> MRGSHHHHHHGSLVPRGSPFVNKQFNYKDPVNGVDIAYIKIPNAGQMQPVKAFKIHNKIWVIPERDTFTNPEEGDLNPPPEAKQVPVSYYDSTYLSTDNEKDNYLKGVTKLFERIYSTDLGRMLLTSIVRGIPFWGGSTIDTELKVIDTNCINVIQPDGSYRSEELNLVIIGPSADIIQFECKSFGHEVLNLTRNGYGSTQYIRFSPDFTFGFEESLEVDTNPLLGAGKFATDPAVTLAHQLIHAGHRLYGIAINPNRVFKVNTNAYYEMSGLEVSFEELRTFGGHDAKFIDSLQENEFRLYYYNKFKDIASTLNKAKSIVGTTASLQYMKNVFKEKYLLSEDTSGKFSVDKLKFDKLYKMLTEIYTEDNFVKFFKVLNAKTFLNFDKAVFKINIVPKVNYTIYDGFNLRNTNLAANFNGQNTEINNMNFTKLKNFTGLFEFYKLLCVRGIITSKTKSLDKGYNKALNDLCIKVNNWDLFFSPSEDNFTNDLNKGEEITSDTNIEAAEENISLDLIQQYYLTFNFDNEPENISIENLSSDIIGQLELMPNIERFPNGKKYELDKYTMFHYLRAQEFEHGKSRIALTNSVNEALLNPSRVYTFFSSDYVKKVNKATEAAMFLGWVEQLVYDFTDETSEVSTTDKIADITIIIPYIGPALNIGNMLYKDDFVGALIFSGAVILLEFIPEIAIPVLGTFALVSYIANKVLTVQTIDNALSKRNEKWDEVYKYIVTNWLAKVNTQIDLIRKKMKEALENQAEATKAIINYQYNQYTEEEKNNINFNIDDLSSKLNESINKAMININKFLNQCSVSYLMNSMIPYGVKRLEDFDASLKDALLKYIYDNRGTLIGQVDRLKDKVNNTLSTDIPFQLSKYVDNQRLLSTFTEYIKNIINTSILNLRYESNHLIDLSRYASKINIGSKVNFDPIDKNQIQLFNLESSKIEVILKNAIVYNSMYENFSTSFWIRIPKYFNSISLNNEYTIINCMENNSGWKVSLNYGEIIWTLQDTQEIKQRVVFKYSQMINISDYINRWIFVTITNNRLNNSKIYINGRLIDQKPISNLGNIHASNNIMFKLDGCRDTHRYIWIKYFNLFDKELNEKEIKDLYDNQSNSGILKDFWGDYLQYDKPYYMLNLYDPNKYVDVNNVGIRGYMYLKGPRGSVMTTNIYLNSSLYRGAKFIIKKYASGNKDNIVRNNDRVYINVVVKNKEYRLATNASQAGVEKILSALEIPDVGNLSQVVVMKS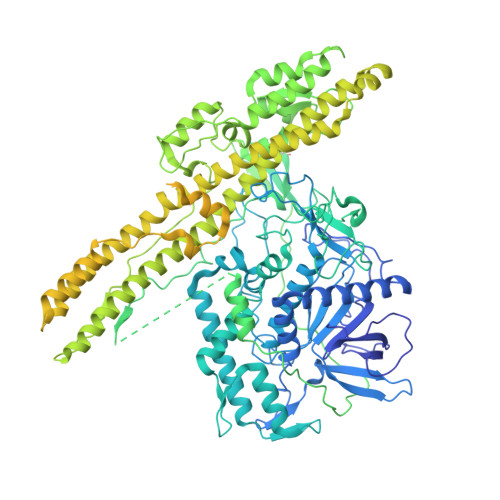KNDQGITNKCKMNLQDNNGNDIGFIGFHQFNNIAKLVASNWYNRQIERSSRTLGCSWEFIPVDDGWGERPLVPPTPGSAWSHPQFEK> ELTPDQQTLLHFIMDSYNKQRMPQEITNKILKEEFSAEENFLILTEMATNHVQVLVEFTKK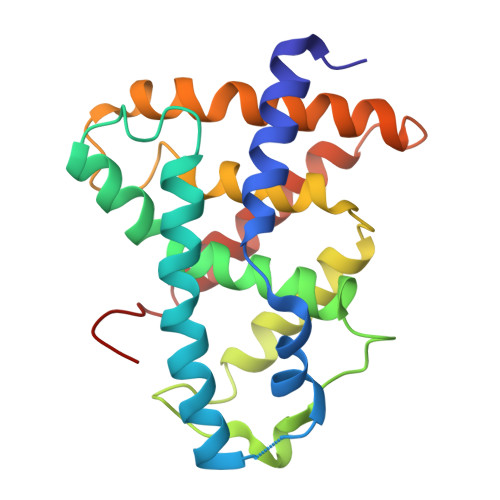LPGFQTLDHEDQIALLKGSAVEAMFLRSAEIFNKKLPSGHSDLLEERIRNSGISDEYITPMFSFYKSIGELKMTQEEYALLTAIVILSPDRQYIKDREAVEKLQEPLLDVLQKLCKIHQPENPQHFACLLGRLTELRTFNHHHAEMLMSW>MSASAQQLAEELQIFGLDCEEALIEKLVELCVQYGQNEEGMVGELIAFCTSTHKVGLTSEILNSFEHEFLSKRLSKARHSTCKDSGHAGARDIVSIQELIEVEEEEEILLNSYTTPSKGSQKRAISTPETPLTKRSVSTRSPHQLLSPSSFSPSATPSQKYNSRSNRGEVVTSFGLAQGVSWSGRGGAGNISLKVLGCPEALTGSYKSMFQKLPDIREVLTCKIEELGSELKEHYKIEAFTPLLAPAQEPVTLLGQIGCDSNGKLNNKSVILEGDREHSSGAQIPVDLSELKEYSLFPGQVVIMEGINTTGRKLVATKLYEGVPLPFYQPTEEDADFEQSMVLVACGPYTTSDSITYDPLLDLIAVINHDRPDVCILFGPFLDAKHEQVENCLLTSPFEDIFKQCLRTIIEGTRSSGSHLVFVPSLRDVHHEPVYPQPPFSYSDLSREDKKQVQFVSEPCSLSINGVIFGLTSTDLLFHLGAEEISSSSGTSDRFSRILKHILTQRSYYPLYPPQEDMAIDYESFYVYAQLPVTPDVLIIPSELRYFVKDVLGCVCVNPGRLTKGQVGGTFARLYLRRPAADGAERQSPCIAV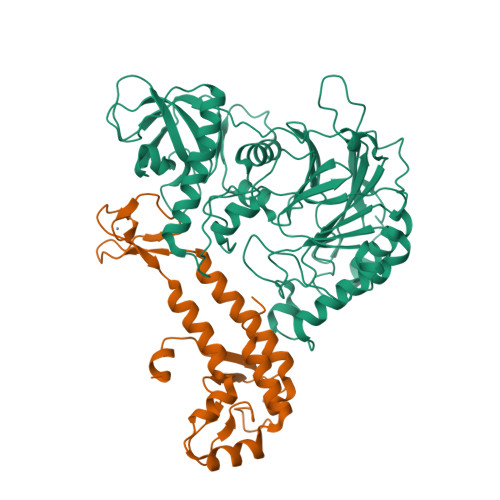QVVRI[4x];>AQLTDEEKYRDCERFKCPCPTCGTENIYDNVFDGSGTDMEPSLYRCSNIDCKASPLTFTVQLSNKLIMDIRRFIKKYYDGWLICEEPTCRNRTRHLPLQFSRTGPLCPACMKATLQPEYSDKSLYTQLCFYRYIFDAECALEKLTTDHEKDKLKKQFFTPKVLQDYRKLKNTAEQFLSRS[4x]>YEQKVRPCIDLIDSLRALGVEQDLALPAIAVIGDQSSGKSSVLEALSGVALPRGSGIVTRCPLVLKLKKQPCEAWAGRISYRNTELELQDPGQVEKEIHKAQNVMAGNGRGISHELISLEITSPEVPDLTIIDLPGITRVAVDNQPRDIGLQIKALIKKYIQRQQTINLVVVPCNVDIATTEALSMAHEVDPEGDRTIGILTKPDLMDRGTEKSVMNVVRNLTYPLKKGYMIVKCRGQQEITNRLSLAEATKKEITFFQTHPYFRVLLEEGSATVPRLAERLTTELIMHIQKSLPLLEGQIRESHQKATEELRRCGADIPSQEADKMFFLIEKIKMFNQDIEKLVEGEEVVRENETRLYNKIREDFKNWVGILATNTQKVKNIIHEEVEKYEKQYRGKELLGFVNYKTFEIIVHQYIQQLVEPALSMLQKAMEIIQQAFINVAKKHFGEFFNLNQTVQSTIEDIKVKHTAKAENMIQLQFRMEQMVFCQDQIYSVVLKKVREEIFNPLGTPSQNMKLNSH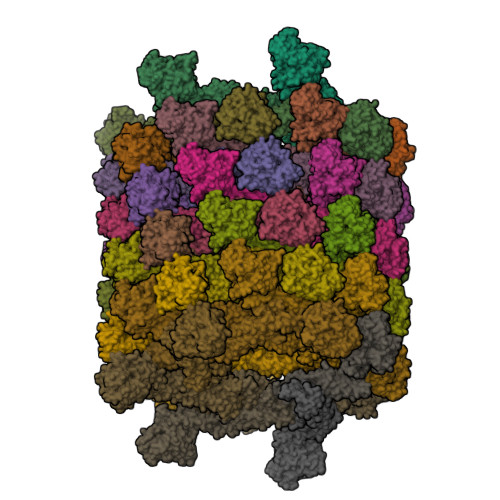FPSNESSVSSFTEIGIHLNAYFLETSKRLANQIPFIIQYFMLRENGDSLQKAMMQILQEKNRYSWLLQEQSETATKRRILKERIYRLTQARHALCQFSS[62x]>[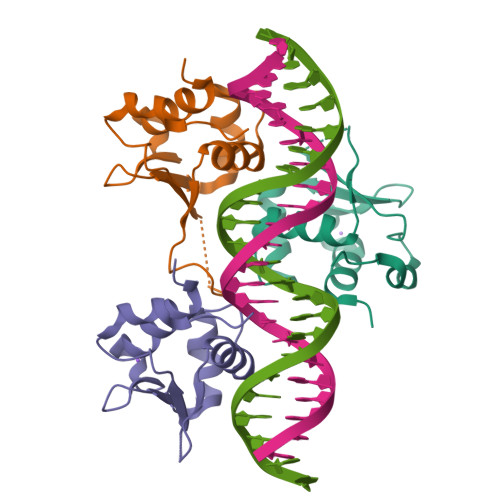6x]GHHHHHHVPAFLTKLWTLVSDPDTDALICWSPSGNSFHVFDQGQFAKEVLPKYFKHNNMASFVRQLNMYGFRKVVHIEQGGLVKPERDDTEFQHPCFLRGQEQLLENIKRKVT>MKLSARNQLAGKVVSIKEGAVNGIVVLDIGGGNQISSTISMDSIRELGLQVGSDAYAVIKATSVM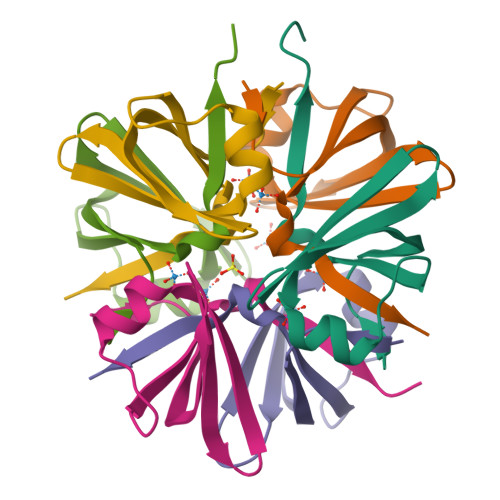IGIDDWS[6x]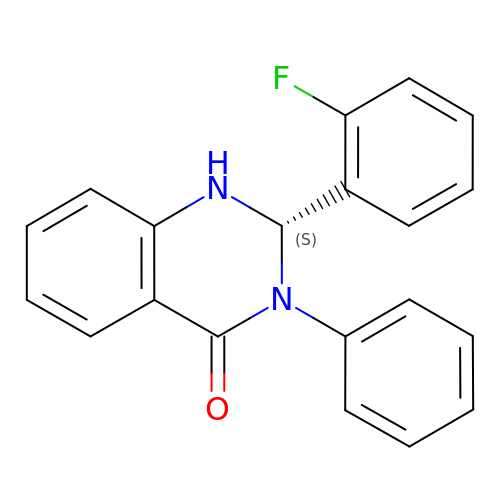(2S)-2-(2-fluorophenyl)-3-phenyl-1,2-dihydroquinazolin-4-one | C20 H15 F N2 O | UMMDFHVNOCVOCD-IBGZPJMESA-N>[2x]MMFGKKKNNGGSSTARYSAGNKYNTLSNNYALSAQQLLNASKIDDIDSMMGFERYVPPQYNGRFDAKDIDQIPGRVGWLTNMHATLVSQETLSSGSNGGGNSNDGERVTTNQGISGVDFYFLDEEGGSFKSTVVYDPYFFIACNDESRVNDVEELVKKYLESCLKSLQIIRKEDLTMDNHLLGLQKTLIKLSFVNSNQLFEARKLLRPILQDNANNNVQRNIYNVAANGSEKVDAKHLIEDIREYDVPYHVRVSIDKDIRVGKWYKVTQQGFIEDTRKIAFADPVVMAFAIATTKPPLKFPDSAVDQIMMISYMIDGEGFLITNREIISEDIEDFEYTPKPEYPGFFTIFNENDEVALLQRFFEHIRDVRPTVISTFNGDFFDWPFIHNRSKIHGLDMFDEIGFAPDAEGEYKSSYCSHMDCFRWVKRDSYLPQGSQGLKAVTQSKLGYNPIELDPELMTPYAFEKPQHLSEYSVSDAVATYYLYMKYVHPFIFSLCTIIPLNPDETLRKGTGTLCEMLLMVQA;>[2x]MSINLHSAPEYDPSYKLIQLTPELLDIIQDPVQNHQLRFKSLDKDKSEVVLCSHDKTWVLKQRKHSNTVLLMREFVPEQPITFDETLLFGLSKPYMDVVGFAKTESEFETRETHGELNLNSVPIYNGELDFSDKIMKRSSTKVIGTLEELLENSPCSALEGISKWHKIGGSVKDGVLCILSQDFLFKALHVLLMSAMAESLDLQHLNVEDTHHAVGKDIEDEFNPYTREIIETVLNKFAVQEQEAENNTWRLRIPFIAQWYGIQALRKYVSGISMPIDEFLIKWKSLFPPFFPCDIDIDMLRGYHFKPTDKTVQYIAKSTLPMDPKERFKVLFRLQSQWDLEDIKPLIEELNSRGMKIDSFIMKYARRKRLGKKTVVTSR;>[2x]MPSVDIDASQWQKLTQSREKQTTVITPLG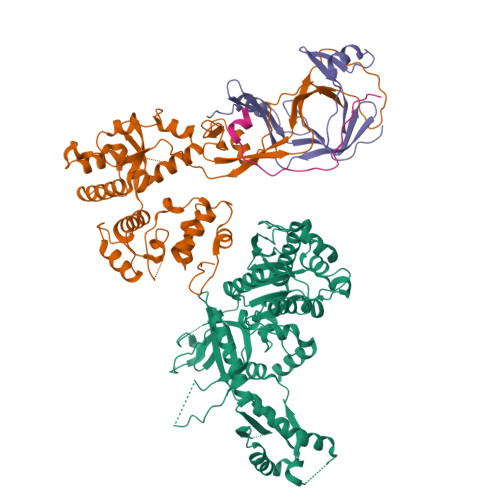MMMLEIQGELELPKDFASLARRDSPNEGRFSEQDGETLIRFGSLQIDGERATLFVGKKQRLLGKVTKLDVPMGIMHFNSKDNKVELVDVMKYKVIFKDRPLPIM;>TVKIWVKYNEGFSNAVRKNVTWNNLW[2x]> GAMVQISEVRGNTRDHRTAAHTHIKGLGLNSSGIAEKQAAGFVGQCAAREACGVVVDLIKAHKMAGRGVLLAGGPGTGKTALALAISQELGTKIPFCPITGSEIYSTEVKKTEVLMENFRRAIGLRVRETKDVYEGEVTEMTPEEAENPLGGYGKTISTLLIGLKSARGQKKLRLDPSI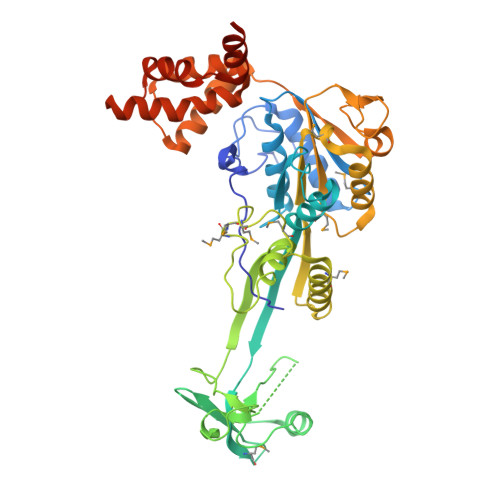YEAIQKERVQVGDVIYIETNTGACKRVGRSDAYATEFDLEAEEYVPIPKGEVHKKKEIVQDVTLHDLDVANARPQGGQDIISMMGQLMKPKMTEITDKLRMEINKVVQKYINQGVAELIPGVLFIDEAHMLDIECFTYLNKALESPIAPIVVLASNRGIATIRGADDLKAAHGIPPDFLQRLLIIPTHPYEPDEIRRIVRIRAQTEGVQLTDAAVDRVAEHGVRISLRYCLQLLAPASILARVNGRTQVDVQDIAEAEELFLDARRSANILTSTGESGGLHGFIS>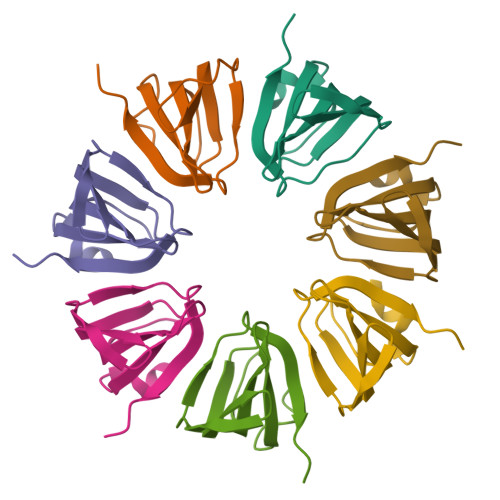[7x]MHHHHHHMSESSDISAMQPVNPKPFLKGLVNHRVGVKLKFNSTEYRGTLVSTDNYFNLQLNEAEEFVAGVSHGTLGEIFIRCNNVLYIRELPN(1S)-2-[(2S,5R)-2-(AMINOMETHYL)-5-ETHYNYLPYRROLIDIN-1-YL]-1-CYCLOPENTYL-2-OXOETHANAMINE 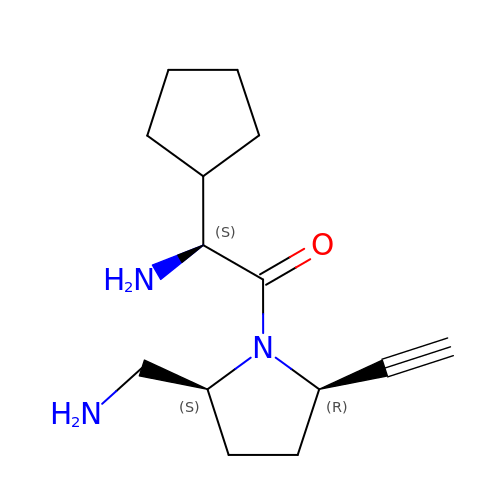| C14 H23 N3 O | XYVMJMYCUZCIPB-AVGNSLFASA-N>[2x]STHETNALHFMFNQFSKDQKDLILQGDATTGTDGNLELTRVSSNGSPQGSSVGRALFYAPV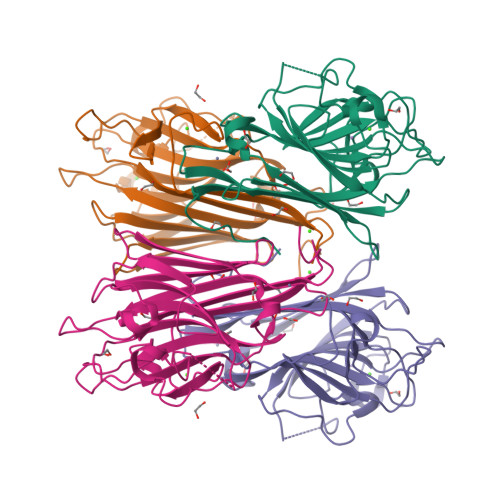HIWESSAVVASFEATFTFLIKSPDSHPADGIAFFISNIDSSIPSGSTGRLLGLFPDANVIRNSTTIDFNAAYNADTIVAVELDTYPNTDIGDPSYPHIGIDIKSVRSKKTAKWNMQNGKVGTAHIIYNSVDKRLSAVVSYPNADSATVSYDVDLDNVLPEWVRVGLSASTGLYKETNTILSWSFTSKLKSNEIPDIATVV> MEFKKVAKETAITLQSYLTYQAVRLISQQLSETNPGQAIWLGEFSKRHPIQESDLYLEAMMLENKELVLRILT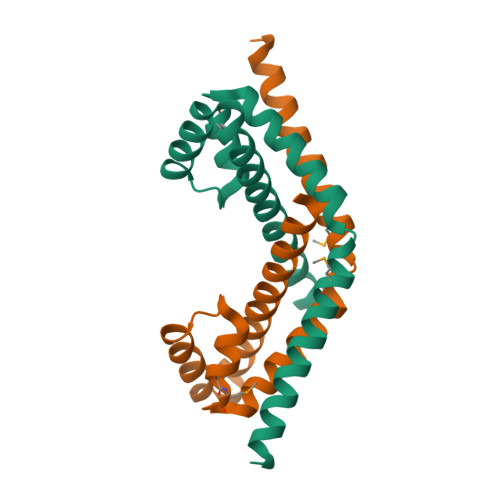VRENLAEGVLEFLPEMVLSQIKQSNGNHRRSLLERLTQVDSSSTDQTEPNPGESDTSEDSE> MAKDIEISASESKFILEALRQNYRLDGRSFDQFRDVEITFGKEFGDVSVKMGNTKVHCRISCQIAQPYEDRPFEGLFVISTEISPMAGSQFENGNITGEDEVLCSRIIEKSVRRSGALDVEGLCIVAGSKCWAVRADVHFLDCDGGFIDASCIAVMAGLMHFKKPDITVHGEQIIVHPVNEREPVPLGILHIPICVTFSFFNPQDTEENIKGETNSEISIIDATLKEELLRDGVLTVTLNKNREVVQVSKAGGLPMDALTLMKCCHEAYSIIEKITDQILQLLKEDSEKRNKYAAMLTSENAREI;> GPDHMSRLEIYSPEGLRLDGRRWNELRRFESSINTHPHAADGSSYMEQGNNKIITLVKGPKEPRLKSQMDTSKALLNVSVNITKFSKFERSKSSHKNERRVLEIQTSLVRMFEKNVMLNIYPRTVIDIEIHVLEQDGGIMGSLINGITLALIDAGISMFDYISGISVGLYDTTPLLDTNSLEENAMSTVTLGVVGKSEKLSLLLVEDKIPLDRLENVLAIGIAGAHRVRDLMDEELRKHAQKRVSNASAR;> MAESTTLETIEIHPITFPPEVLARISPELSLQRHLSLGIRPCLRKYEEFRDVAIENNTLSRYADAGNIDTKNNILGSNVLKSGKTIVITSITGGIIEETSAAIKDLDDFGEEELFEVTKEEDIIANYASVYPVVEVERGRVGACTDEEMTISQKLHDSILHSRILPKKALKVKAGVRSANEDGTFSVLYPDELEDDTLNETNLKMKRKWSYVLYAKIVVLSRTGPVFDLCWNSLMYALQSVKLPRAFIDERASDLRMTIRTRGRSATIRETYEIICDQTKSVPLMINAKNIAFASNYGIVELDPECQLQNSDNSEEEEVDIDMDKLNTVLIADLDTEAEETSIHSTISILAAPSGNYKQLTLVGGGAKITPEMIKRSLLLSRVRADDLSTRFNI;> GSMSVQAEIGILDHVDGSSEFVSQDTKVICSVTGPIEPKARQELPTQLALEIIVRPAKGVATTREKVLEDKLRAVLTPLITRHCYPRQLCQITCQILESGEDEAEFSLRELSCCINAAFLALVDAGIALNSMCASIPIAIIKDTSDIIVDPTAEQLKISLSVHTLALEFVNGGKVVKNVLLLDSNGDFNEDQLFSLLELGEQKCQELVTNIRRIIQDNISPRLVV;> GDPHMSLSVAEKSYLYDSLASTPSIRPDGRLPHQFRPIEIFTDFLPSSNGSSRIIASDGSECIVSIKSKVVDHHVENELLQVDVDIAGQRDDALVVETITSLLNKVLKSGSGVDSSKLQLTKKYSFKIFVDVLVISSHSHPVSLISFAIYSALNSTYLPKLISAFDDLEVEELPTFHDYDMVKLDINPPLVFILAVVGNNMLLDPAANESEVANNGLIISWSNGKITSPIRSVALNDSNVKSFKPHLLKQGLAMVEKYAPDVVRSLENL;> MNVQDRRRLLGPAAAKPMAFSNTTTHVPEKKSTDLTPKGNESEQELSLHTGFIENCNGSALVEARSLGHQTSLITAVYGPRSIRGSFTSQGTISIQLKNGLLEKYNTNELKEVSSFLMGIFNSVVNLSRYPKSGIDIFVYLTYDKDLTNNPQDDDSQSKMMSSQISSLIPHCITSITLALADAGIELVDMAGAGEANGTVVSFIKNGEEIVGFWKDDGDDEDLLECLDRCKEQYNRYRDLMISCLMNQET;> GDPHMSTFIFPGDSFPVDPTTPVKLGPGIYCDPNTQEIRPVNTGVLHVSAKGKSGVQTAYIDYSSKRYIPSVNDFVIGVIIGTFSDSYKVSLQNFSSSVSLSYMAFPNASKKNRPTLQVGDLVYARVCTAEKELEAEIECFDSTTGRDAGFGILEDGMIIDVNLNFARQLLFNNDFPLLKVLAAHTKFEVAIGLNGKIWVKCEELSNTLACYRTIMECCQKNDTAAFKDIAKRQFKEILTVKEE;> GDPHMSEVITITKRNGAFQNSSNLSYNNTGISDDENDEEDIYMHDVNSASKSESDSQIVTPGELVTDDPIWMRGHGTYFLDNMTYSSVAGTVSRVNRLLSVIPLKGRYAPETGDHVVGRIAEVGNKRWKVDIGGKQHAVLMLGSVNLPGGILRRKSESDELQMRSFLKEGDLLNAEVQSLFQDGSASLHTRSLKYGKLRNGMFCQVPSSLIVRAKNHTHNLPGNITVVLGVNGYIWLRKTSQMDLARDTPSANNSSSIKSTGPTGAVSLNPSITRLEEESSWQIYSDENDPSISNNIRQAICRYANVIKALAFCEIGITQQRIVSAYEASMVYSNVGELIEKNVMESIGSDILTAEKMRGNGN;> GDPHMACNFQFPEIAYPGKLICPQYGTENKDGEDIIFNYVPGPGTKLIQYEHNGRTLEAITATLVGTVRCEEEKKTDQEEEREGTDQSTEEEKSVDASPNDVTRRTVKNILVSVLPGTEKGRKTNKYANNDFANNLPKEGDIVLTRVTRLSLQRANVEILAVEDKPSPIDSGIGSNGSGIVAAGGGSGAATFSVSQASSDLGETFRGIIRSQDVRSTDRDRVKVIECFKPGDIVRAQVLSLGDGTNYYLTTARNDLGVVFARAANGAGGLMYATDWQMMTSPVTGATEKRKCAKPF;> SLMVEKPQLKFKSPIDNSESHPFIPLLKEKPNALKPLSESLRLVDDDENNPSHYPHPYEYEIDHQEYSPEILQIREEIPSKSWDDSVPIWVDTSTELESMLEDLKNTKEIAVNLEHHDYRSYYGIVCLMQISTRERDYLVDTLKLRENLHILNEVFTNPSIVKVFHGAFMDIIWLQRDLGLYVVGLFDTYHASKAIGLPRHSLAYLLENFANFKTSKKYQLADWRIRPLSKPMTAYARADTHFLLNIYDQLRNKLIESNKLAGVLYESRNVAKRRFEYSKYRPLTPSSEVYSPIEKESPWKILMYQYNIPPEREVLVRELYQWRDLIARRDDESPRFVMPNQLLAALVAYTPTDVIGVVSLTNGVTEHVRQNAKLLANLIRDALRN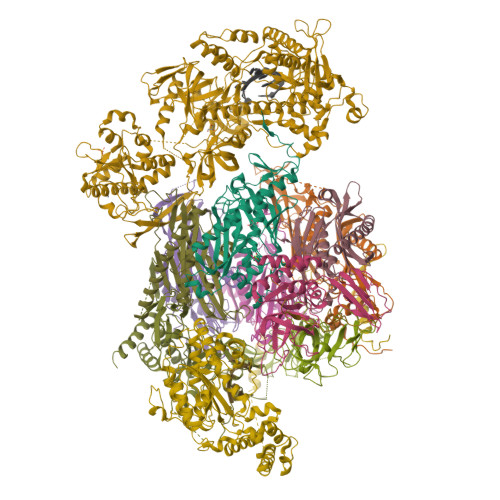IKNTNEEATPIPSSETKADGILLETISVPQIRDVMERFSVLCNSNISKSRAKPVTNSSILLGKILPREEHDIAYSKDGLPNKVKTEDIRIRAQNFKSALANLEDIIFEIEKPLVVPVKLEEIKTVDPASAPNHSPEIDNLDDLVVLKKKNIQKKQPAKEKGVTEKDAVDYSKI;> SLMSVPAIAPRRKRLADGLSVTQKVFVRSRNGGATKIVREHYLRSDIPCLSRSCTKCPQIVVPDAQNELPKFILSDSPLELSAPIGKHYVVLDTNVVLQAIDLLENPNCFFDVIVPQIVLDEVRNKSYPVYTRLRTLCRDSDDHKRFIVFHNEFSEHTFVERLPNETINDRNNRAIRKTCQWYSEHLKPYDINVVLVTNDRLNREAATKEVESNIITKSLVQYIELLPNADDIRDSIPQMDSFDKDLERDTFSDFTFPEYYSTARVMGGLKNGVLYQGNIQISEYNFLEGSVSLPRFSKPVLIVGQKNLNRAFNGDQVIVELLPQSEWKAPSSIVLDSEHFDVNDNPDIEAGDDDDNNESSSNTTVISDKQRRLLAKDAMIAQRSKKIQPTAKVVYIQRRSWRQYVGQLAPSSVDPQSSSTQNVFVILMDKCLPKVRIRTRRAAELLDKRIVISIDSWPTTHKYPLGHFVRDLGTIESAQAETEALLLEHDVEYRPFSKKVLECLPAEGHDWKAPTKLDDPEAVSKDPLLTKRKDLRDKLICSIDPPGCVDINDALHAKKLPNGNWEVGVHIADVTHFVKPGTALDAEGAARGTSVYLVDKRIDMLPMLLGTDLCSLKPYVDRFAFSVIWELDDSANIVNVNFMKSVIRSREAFSYEQAQLRIDDKTQNDELTMGMRALLKLSVKLKQKRLEAGALNLASPEVKVHMDSETSDPNEVEIKKLLATNSLVEEFMLLANISVARKIYDAFPQTAMLRRHAAPPSTNFEILNEMLNTRKNMSISLESSKALADSLDRCVDPEDPYFNTLVRIMSTRCMMAAQYFYSGAYSYPDFRHYGLAVDIYTHFTSPIRRYCDVVAHRQLAGAIGYEPLSLTHRDKNKMDMICRNINRKHRNAQFAGRASIEYYVGQVMRNNESTETGYVIKVFNNGIVVLVPKFGVEGLIRLDNLTEDPNSAAFDEVEYKLTFVPTNSDKPRDVYVFDKVEVQVRSVMDPITSKRKAELLLK;> GSVKRVVYKKRPNLIISNVGYSELRKPEGVISGRKTFGDNSD> PRKARTA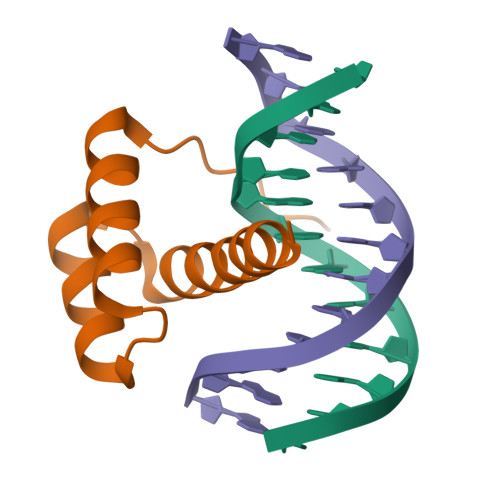FSDHQLNQLERSFERQKYLSVQDRMDLAAALNLTDTQVKTWYQNRRTKWKRQTAV> MLSRASIRAYSSIPNSVKIAAKESATDLTKLSVIINNAGSKTGKSGVSHLLSKFTFLNNGAKSALRFTRESELLGGTFESKVTRDALILNTTFLKQDLPYYVEALGNVVSNTQFAPHEFNEIVLPTANAETKLANANPAFKGVEKLHEITFRRGLGNPLFYNESTPIKLEEVAQFSKEQFSGENISIVAEGANEEDLTKFVSESAFCYLPSSSSNGAKALPTNTFTGQEARV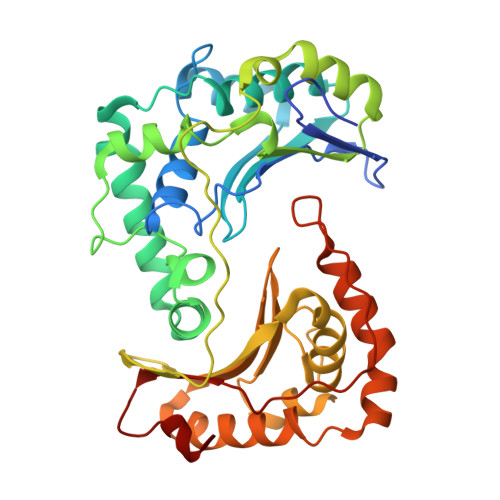PSSGASSALIGIPVKPADFGKYEVLSAAIGTSTLPSTSTPLAQIPGATSHLYKYQDAGLFVISVSGEASQVAQGIKQAKSVAESVSSSALSEAVKAAELSVALQSTVDSPLNVKVVAEEAPISKFNYVAVGDLDVLPYADEL5'-O-[(R)-hydroxy{[(2E)-3-(5-methoxy-4-oxocyclohexa-1,5-dien-1-yl)prop-2-enoyl]oxy}phosphoryl]adenosine 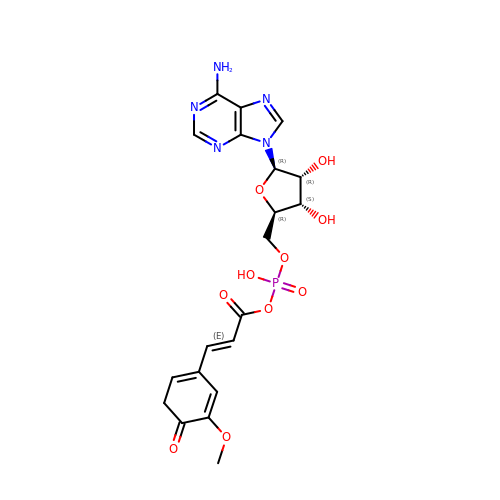| C20 H22 N5 O10 P | DTAKVQMQJSRZPC-NLGGRGNSSA-N>[2x]MRSRRVDVMDVMNRLILAMDLMNRDDALRVTGEVREYIDTVKIGYPLVLSEGMDIIAEFRKRFGCRIIADFKVADIPETNEKICRATFKAGADAIIVHG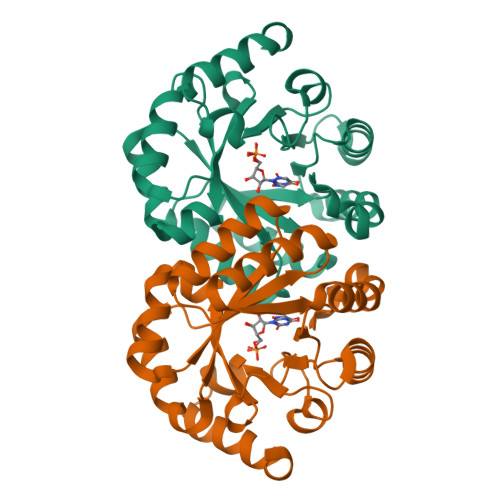FPGADSVRACLNVAEEMGREVFLLTEMAHPGAEMFIQGAADEIARMGVDLGVKNYVGPSTRPERLSRLREIIGQDSFLISPGVGAQGGDPGETLRFADAIIVGRSIYLADNPAAAAAGIIESIKDLLNP> MGYYDIDDVLADGTEFPCKFQYDIPGLGYLENNPGRPITKNTKLSLPLWLARILAIVGGDEALVDEEPVPFVELLPPDMFSTKVMNAIKTDPVALDLHSINSHFFSLAIKWIMLFSEKELANVVSELLLQRAQELN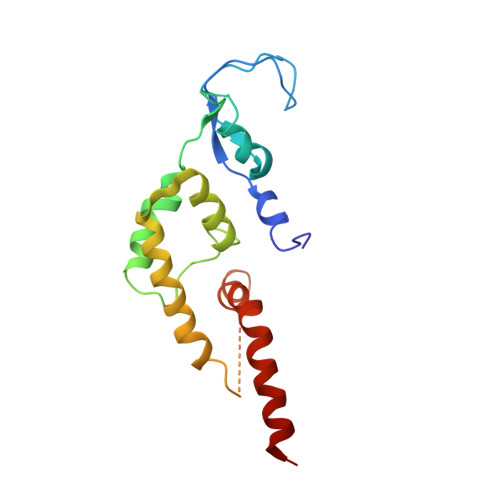HHASSLSIDLNADSTGKNSANTNIATSTFLLKLEEMEKEIYKKSHESYKDTKRWMFKK> MRRRAVLGGAVVYPEGPPPSYESVMQQQAAMIQPPLEAPFVPPRYLAPTEGRNSIRYSELSPLYDTTKLYLVDNKSADIASLNYQNDHSNFLTTVVQNNDFTPTEASTQTINFDERSRWGGQLKTIMHTNMPNVNEYMFSNKFKARVMVSRKAPEGVTVNDTYDHKEDILKYEWFEFILPEGNFSATMTIDLMNNAIIDNYLEIGRQNGVLESDIGVKFDTRNFRLGWDPETKLIMPGVYTYEAFHPDIVLLPGCGVDFTESRLSNLLGIRKRHPFQEGFKIMYEDLEGGNIPALLDVTAYEESKKDTTTETTTKKELKIQPLEKDSKSRSYNVLEDKINTAYRSWYLSYNYGNPEKGIRSWTLLTTSDVTCGAEQVYWSLPDMMQDPVTFRSTRQVNNYPVVGAELMPVFSKSFYNEQAVYSQQLRQATSLTHVFNRFPENQILIRPPAPTITTVSENVPALTDHGTLPLRSSIRGVQRVTVTDARRRTCPYVYKALGIVAPRVLSSR;> MKRARPSEDTFNPVYPYDTEC

Dodecahedron-base is a small icosahedral virus-like particle composed of 12 copies of the Ad3 pentameric Pb protein and is capable of efficient cell entry. Virus-like particles, called dodecahedron-fiber (DF), are generated during the adenovirus serotype 3 (Ad3) life cycle in infected cells. These symmetrical, dodecahedral particles are composed of 12 copies of the viral penton complex, which comprises the pentameric penton base (Pb) and the attached trimeric fiber, both of which are essential for viral cell entry. Through careful examination of the crystal structure, it was determined that residues 48–61 of Ad3 Pb, the Dd building blocks, interlock within the particle through strand-swapping. The strand-swapping considerably increases the contacts between neighboring Pb pentamers which otherwise associates only through three small loop regions.

An orthorhombic crystal form for Ad3 Dd was obtained in the presence of an N-terminal peptide derived from the Ad2/3 fiber consensus sequence. This crystal form contains one full Dd (i.e. 60 copies of the Pb monomer) in the asymmetric unit and therefore allows improvement of the electron density by 60-fold non-crystallographic averaging. Using strict 60-fold non-crystallographic symmetry, the structure has been refined to 3.8 Å resolution (Rfree = 0.280). Additional electron density, corresponding to the sequence NPVYPYDTEC, was visible in the fiber peptide-binding site of the Pb, confirming that the highly conserved FNPVYPY motif of the fiber mediates the binding as previously described. In addition, the conformation of residues 452 to 467 of the Ad3 Pb corresponds to that observed for Ad2 Pb when bound to the fiber peptide (pdb entry 1×9t, ). In both Ad3 Dd crystal forms, the visible electron density for the Pb peptide chain starts at residue Pro48, while a very strong positive electron density (>10 σ and >18 σ, respectively for each crystal form) is consistently present in averaged Fo-Fc maps on the Pb 5-fold axis and coordinated by Glu451 from each subunit. As Ca2+ was present during the crystallization, it is most likely that this density corresponds to a bound calcium ion. Due to methodological limitations it cannot be excluded that non strand-swapped dimers are present in low proportion (<30%) in either crystal form, however the strand swapped form dominates.> GAGAYAYKTIKEDQKRYNERVMGLGLSPEEKQRRAIASATEGGSVPQIRAPSHVPFLLIGGGTAAFAAARSIRARDPGARVLIVSEDPELPYMRPPLSKELWFSDDPNVTKTLQFRQWNGKERSIYFQPPSFYVSAQDLPNIENGGVAVLTGKKVVHLDVRGNMVKLNDGSQITFEKCLIATGGTPRSLSAIDRAGAEVKSRTTLFRKIGDFRALEKISREVKSITVIGGGFLGSELACALGRKSQASGIEVIQLFPEKGNMGKILPQYLSNWTMEKVKREGVKVMPNAIVQSVGVSGGRLLIKLKDGRKVETDHIVTAVGLEPNVELAKTGGLEIDSDFGGFRVNAELQARSNIWVAGDAACFYDIKLGRRRVEHHDHA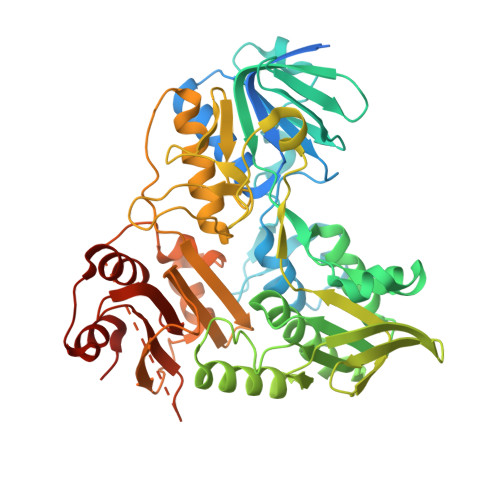VVSGRLAGENMTGAAKPYWHQSMFWSDLGPDVGYEAIGLVDSSLPTVGVFAKATAQDNPKSATEQSGTGIRSESETESEASEITIPPSAPAVPQVPVEGEDYGKGVIFYLRDKVVVGIVLWNVFNRMPIARKIIKDGEQHEDLNEVAKLFNIHED>[2x]MAPVKVFGPAMSTNVARVTLCLEEVGAEYEVVNIDFNTMEHKSPEHLARNPFGQIPAFQDG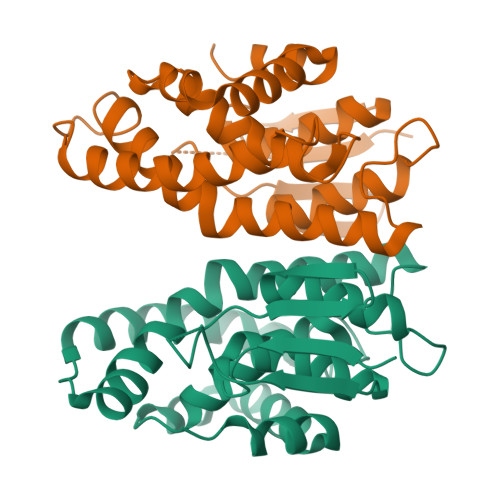DLLLWESRAISKYVLRKYKTDEVDLLREGNLKEAAMVDVWTEVDAHTYNPALSPIVYECLINPLMRGLPTNQTVVDESLEKLKKVLEVYEARLSQHKYLAGDFVSFADLNHFPYTFYFMATPHAALFDSYPHVKAWWDRLMARPAVKKIAATMVPPKAHHHHHH> SMPFPKDCSQAMLNGDTTSGLYTIYLNGDKAQALEVFCDMTSDGGGWIVFLRRKNGRENFYQNWKAYAAGFGDRREEFWLGLDNLNKITAQGQYELRVDLRDHGETAFAVYDKFSVGDAKTRYKLKVEGYSGTAGDSMAYHNGRSFSTFDKDTDSAITNCALSYKGAFWYRNCHRVNLMGRYGDNNHSQGVNWFH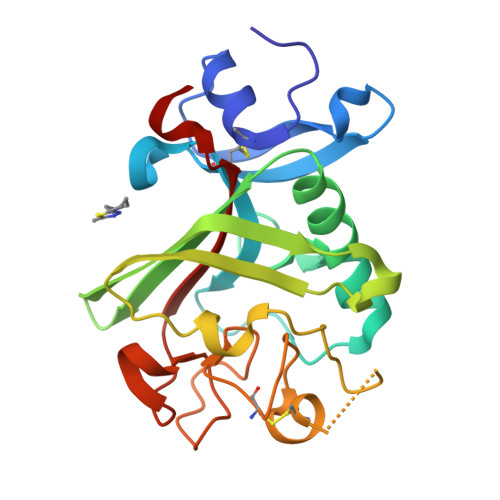WKGHEHSIQFAEMKLRPSNFRNLEG>GVSETAPASRRGELAVCDAVSGWVTDRRTAVDLRGREVEVLGEVPAAGGSPLRQYFFETRCKADNAEEGGPGAGGGGCRGVDRRHWVSECKAKQSYVRALTADAQGRVGWRWIRIDTACVCTLLSRTGR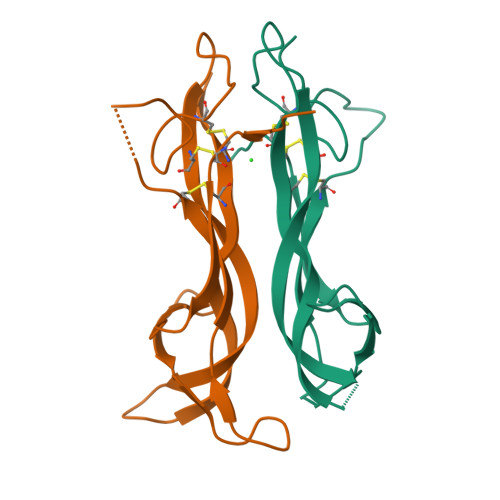A[2x]> MSANNTAKNMHPETRAVGSETSSLQASQDEFENLVRNVDVKSRIMDQYADWKGVRYRLGGSTKKGIDCSGFVQRTFREQFGLELPRSTYEQQEMGKSVSRSNLRTGD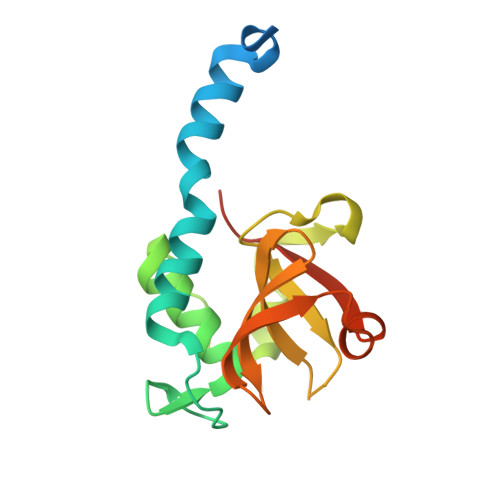LVLFRAGSTGRHVGIYIGNNQFVHASTSSGVIISSMNEPYWKKRYNEARRVLSRSHHHHHH>NKRKDLESKVFKILFESLESTRKAIAKQNQEKWKKYFILAKRKLLLSQKIETELVLEQRDDIDINSLSIASGNESESVFKIYDLCEQLISKIEYQLPQLESQYSQPTDLDYILEDSAMQTLKRLQDEEGWTEHHSAIYRQSIQSMKREVHTDLLLYSSILYDNLIH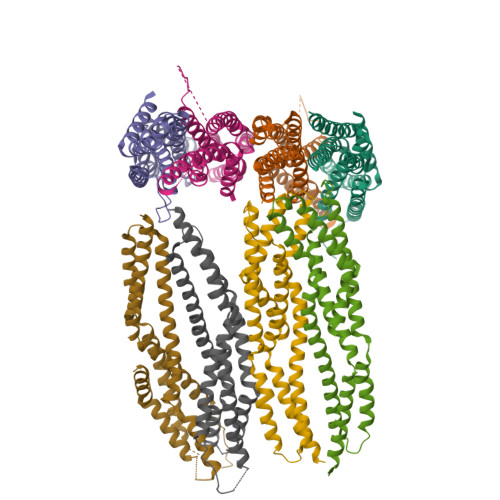DLSIFFYIPREIGNFINNISNPTSLNEANQELLYNMTLGLENLLNGEFDSAMEHYAMDYMKNKVES[8x]> MGSDAFDEMDEIWALYADDGAQALDAMEASLLALQAGEDAAAHVGPLFRAVHTFKGNSRVLGLSVVESRAHLCEDLIGLVRDAGVPMDGEIVEILLFASDTLRAMLEETAASRADVEGTGSEALMDQLRSKIARCSRSHHHHHH;> MRGSHHHHHHGSPYNVMIVDDAAMMRLYIASFIKTLPDFKVVAQAANGQEALDKLAAQPNVDLILLNIEMPVMDGMEFLRHAKLKTRAKICMLASVAVSGSPHAARARELGADGVVAKPSGTVSHDLEEKTGGELARTMRTLMAA

Two-component pathways comprise sensor histidine kinases (HPK) and response regulators (RRs). Once phosphorylated, the HPK transfers the phosphoryl group to an aspartate residue within the receiver domain of the cognate RR. Neither CheA3 nor CheA4 is capable of autophosphorylation; instead, CheA4 phosphorylates CheA3 on H51 of the P1 (Hpt) domain. Once phosphorylated, CheA3-P serves as a specific phosphodonor for the chemotaxis RRs, CheY1, CheY6, and CheB2.

To show that the conclusions drawn from the unphosphorylated structure are also valid for the physiologically relevant, phosphorylated complex, we solved the structure of phosphorylated CheA3P1 in complex with CheY6. Since the rapid rate of phosphotransfer between CheA3P1-P and CheY6 does not allow crystallization of the wild-type, phosphorylated complex, we formed a stable, complex by introducing two substitutions, D56N and S83A, in the active site of CheY6. These substitutions have previously been shown to abolish phosphotransfer from CheA3P1-P. The structure was solved to 2.8 Å by molecular replacement using the unphosphorylated structure as model. The structure shows clear additional density adjacent to Nε2 of His51 of CheA3P1 in agreement with phosphorylation of this residue. Due to the moderate resolution of the analysis, residues 60–65, 85–97, and 111–121 on CheY6 could not be traced and were not included in the final model. Compared to the unphosphorylated complex, CheA3P1-P undergoes a rigid body translation of 2.1 Å relative to the RR. This realignment of CheA3P1-P positions the phosphorylated His51 closer to the phosphoacceptor on CheY6, Asp56. The phosphorylated His51 is facing away from the active site of CheY6; however, a 180° flip of this side chain would put it in near linear geometry and place the phosphoryl group within 4.5 Å of Asp56 of CheY6. The orientation of the phosphorylated His51 seen in the crystal structure is likely caused by the lack of a divalent cation in the metal binding site of the RR leading to electrostatic repulsion from the CheY6 active site. Consistent with this, we find very little change in the total buried surface area between the phosphorylated (605 Å2) and unphosphorylated (530 Å2) structures of CheA3P1 complexed with CheY6.> MTKVDFWPTLKDAYEPLYPQQLEILRQQVVSEGGPTATIQSRFNYAWGLIKSTDVNDERLGVKILTDIYKEAESRRRECLYYLTIGCYKLGEYSMAKRYVDTLFEHERNNKQVGALKSMVEDKIQKETL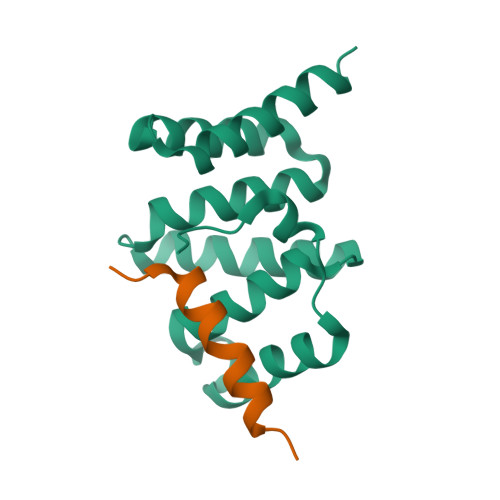;> GSHMDADGKLLTEGGENENLRKNASKKETSLFQGFKSYLPIAELAIENTERLNY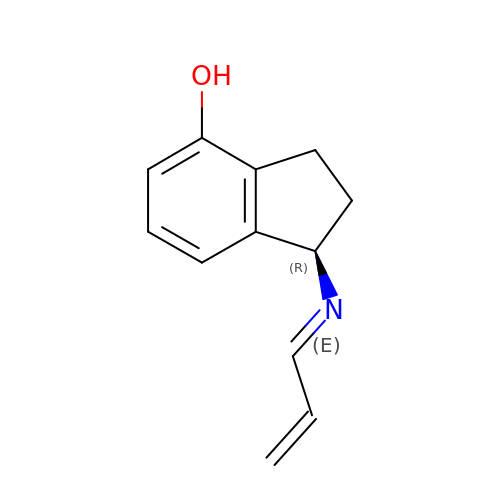4-HYDROXY-N-PROPARGYL-1(R)-AMINOINDAN | C12 H13 N O | OFWOPQIDDNCCLL-KAQJVSAMSA-N>APDTSVSNKQNFSTDVIYQIFTDRFSDGNPANNPTGAAFDGSCTNLRLYCGGDWQGIINKINDGYLTGMGITAIWISQPVENIYSVINYSGVNNTAYHGYWARDFKKTNPAYGTMQDFKNLIDTAHAHNIKVIIDFAPNHTSPASSDDPSFAENGRLYDNGNLLGGYTNDTQNLFHHYGGTDFSTIENGIYKNLYDLADLNHNNSSVDVYLKDAIKMWLDLGVDGIRVDAVKHMPFGWQKSFMATINNYKPVFTFGEWFLGVNEISPEYHQFANESGMSLLDYRFAQKARQVFRDNTDNMYGLKAMLEGSE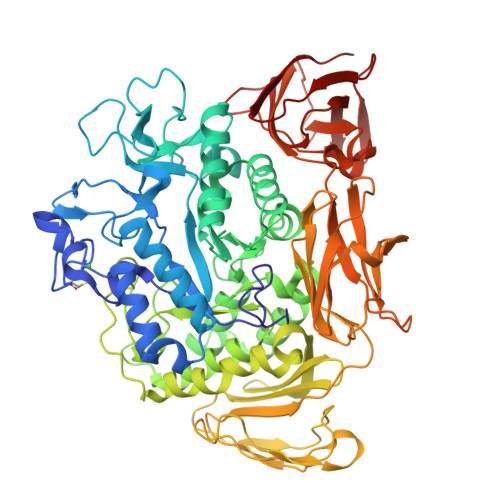VDYAQVNDQVTFIDNHDMERFHTSNGDRRKLEQALAFTLTSRGVPAIYYGSEQYMSGGNDPDNRARLPSFSTTTTAYQVIQKLAPLRKSNPAIAYGSTHERWINNDVIIYERKFGNNVAVVAINRNMNTPASITGLVTSLPRGSYNDVLGGILNGNTLTVGAGGAASNFTLAPGGTAVWQYTTDATTPIIGNVGPMMAKPGVTITIDGRGFGSGKGTVYFGTTAVTGADIVAWEDTQIQVKIPAVPGGIYDIRVANAAGAASNIYDNFEVLTGDQVTVRFVINNATTALGQNVFLTGNVSELGNWDPNNAIGPMYNQVVYQYPTWYYDVSVPAGQTIEFKFLKKQGSTVTWEGGANRTFTTPTSGTATVNVNWQP[2x]5'-[(S)-(3-AMINOPROPYL)(METHYL)-LAMBDA~4~-SULFANYL]-5'-DEOXYADENOSINE | C14 H24 N6 O3 S | 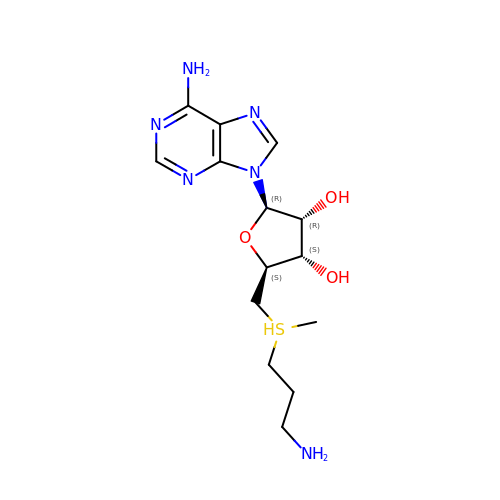KIZZALRCMBIHBH-IDTAVKCVSA-N> SNAIIAGETSIPSQGENMPAYHARPKNADGPLPIVIVVQEIFGVHEHIRDLCRRLAQEGYLAIAPELYFRQGDPNEYHDIPTLFKELVSKVPDAQVLADLDHVASWAARHGGDAHRLLITGFCWGGRITWLYAAHNPQLKAAVAWYGKLVGEKSLNSPKHPVDIAVDLNAPVLGLYGAKDASIPQDTVETMRQALRAANATAEIVVYPEADH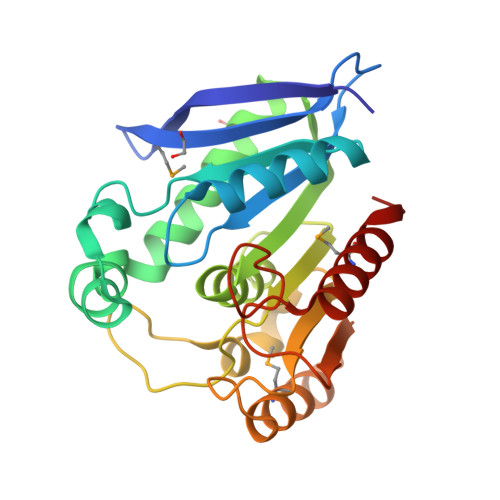AFNADYRASYHEESAKDGWQRMLAWFAQY> GMSFELVAYEKLKGSIRESIITLIKSHNEKAKIIEDKLEYSVKEVSRERQPQVLVLLKTIELLDNSSKEPEDKARVLNALAYYIRDQIAATYKYTSPDNSDFYKSLTISLDLNKDNNPNREDLADMYSALEKFLRSHVYKNSDPRKGYLDKQPFAIKHYSVVDDILELSDRVHKLRHEIIIAARD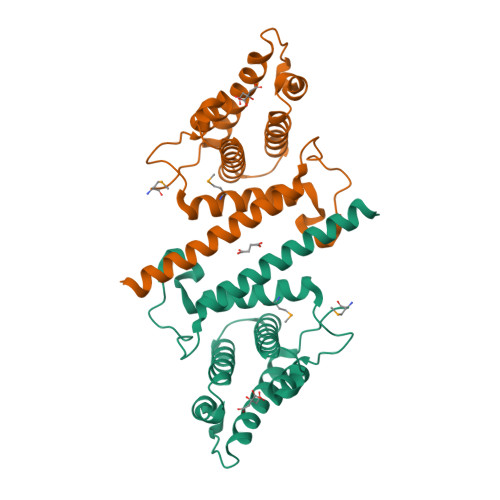LHLLQ6-[3-(3,3-difluoroazetidin-1-yl)prop-1-yn-1-yl]-4-methylpyridin-2-amine | C12 H13 F2 N3 | 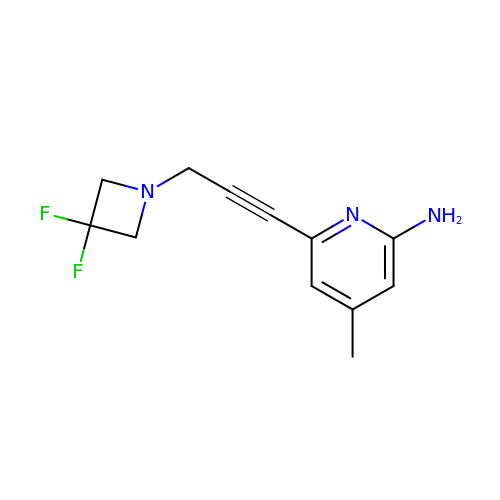OJUWVNWEQOIPOJ-UHFFFAOYSA-N>GPHMTTIEDEDTKVRKQEIIK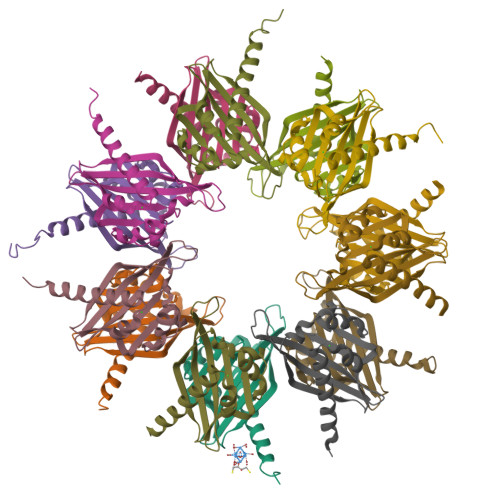VTEQLIEAISNGDFESYTKMCDPGMTAFEPEALGNLVEGLDFHRFYFENLWSRNSKPVHTTILNPHIHLMGDESACIAYIRITQYLDAGGIPRTAQSEETRVWHRRDGKWQIVHFHRSGAPSVLPH[14x]>GAGU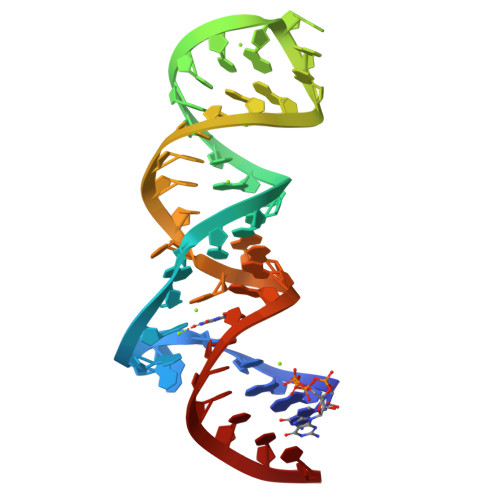AGAAGCGUUCAGCGGCCGAAAGGCCGCCCGGAAAUUGCUCC[2x]>[4x]SNAFLDYGLSEADPDVHAIINKEKDRQFRSLELIASENFTSKAVMEAVGSCLTNKYSEGLPGKRYYGGNEHIDELEILCQQRALAAFHLDGDKWGVNVQPLSGSPANFAVYTAILKPHDRIMGLDLPHGGHLSHGFMTAKRRVSGTSIYFESMPYRLDES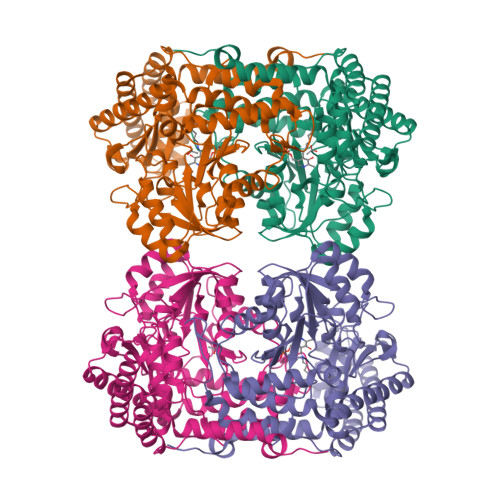TGVIDYDMLEKTAALFRPKLIIAGASAYPRDIDYARFRKIADSVGAFLMMDMAHVSGLIAASVLADPFEFVDIVTTTTHKSLRGPRGGMIFFKKDAVHGVDLESAINNAVFPGLQGGPHNHTIGGLAVCLKYAQSPDFKNYQNQVVANCRALANRLVEHEYKLVSGGSDNHLVLVDLRPSGIDGARVEKILDMASITLNKNSVPGDKSALVPGGIRIGSPAMTTRGLGEKEFELIADLIHEGVRISLEAKSLVSGTKVQDFLNFVLAPEFPLGDKVSNLRRKVEALATQYPIPGV N-Myristoyltransferase (NMT, EC 2.3.1.97) catalyses the transfer of the fatty acid chain C14:0 from myristoyl coenzyme A (MyrCoA) to the N-terminal glycine residue of substrate proteins. This co- and post-translational modification is ubiquitous in eukaryotic organisms and plays a central role in a variety of cellular processes such as the addressing and reversible anchoring of proteins to membranes. In particular, NMT has been validated as a pharmacological target in fungal infections, in a range of parasitic diseases caused by Trypanosoma,7Leishmania8 and Plasmodium protozoa and filarial nematodes, and as a potential target for the treatment of cancer. Herein, we report the synthesis and the structure-guided optimization of a series of quinolines with balanced activity against both Plasmodium vivax and Plasmodium falciparum N-myristoyltransferase (NMT).

First, compound 1 was co-crystallized with PvNMT and S-(2-oxo)pentadecyl-coenzyme A, a non-hydrolysable myristoyl-coenzyme A analogue,26 and the structure of the resulting ternary complex was solved by X-ray crystallography. Overall, 1 adopts a binding mode similar to the original hit compound, 3-butyl-4-((2-cyanoethyl)thio)-6-methoxy-2-methylquinoline (MRT00057965), which we identified in 2012 by high throughput screening. The quinoline fits into a hydrophobic pocket, where it establishes parallel-displaced π–π stacking interactions with the adjacent side-chains of Phe103 and Phe105. The binding of the quinoline ring is reinforced by the establishment of an H-bond between its nitrogen and the hydroxyl function of Ser319. Additionally, the nitrile function of the 2-cyanoethylthioether chain appears to interact with the imidazole ring of His213 (distance ∼3.0 Å). The ligand is modelled bound to the protein at half maximal occupancy due to the low affinity of binding. This is mirrored in the two orientations of residues His213 and Tyr211, corresponding to the bound and free forms. Interestingly, the ester function, introduced to improve the solubility and log P of the hit compound, also establishes polar interactions with PvNMT, through water-mediated H-bonds. The X-ray structure of the complex between 1 and PvNMT shows that a cluster of water molecules surrounds the sulfur atom of the thioether chain. Superposition of the three quinoline–PvNMT complexes present in the asymmetric unit of the crystal shows that the ethyl ester group is flexible and able to adopt different conformations in a relatively large pocket, suggesting that the ethyl chain is suboptimal and that the enzyme may tolerate larger substituents.

>[3x]IDYKFWYTQPVPKINDEFNESVNEPFISDNKVEDVRKDEYKLPPGYSWYVCDVKDEKDRSEIYTLLTDNYVEDDDNIFRFNYSAEFLLWALTSPNYLKTWHIGVKYDASNKLIGFISAIPTDICIHKRTIKMAEVNFLCVHKTLRSKRLAPVLIKEITRRINLENIWQAIYTAGVYLPKPVSDARYYHRSINVKKLIEIGFSSLNSRLTMSRAIKLYRVEDTLNIKNMRLMKKKDVEGVHKLLGSYLEQFNLYAVFTKEEIAHWFLPIENVIYTYVNEENGKIKDMISFYSLPSQILGNDKYSTLNAAYSFYNVTTTATFKQLMQDAILLAKRNNFDVFNALEVMQNKSVFEDLKFGEGDGSLKYYLYNWKCASFAPAHVGIVLL>GATSCIQDEALNSEAAIDACTGDDVQLANINADSKLINVYVNKGADLSKQKLEFVIPEGATIKINDQVAGDTEATYDFSEETHSRKFTVTSEDGQWKPVYTVKVVLAELPTSFNFEELLPSNDYDIFYEFQPGTSQEISKVLQWSSGNPGFKLTGMANSKTDYPTVQVANGFRGKGVKLETRDTGSFGAMVKMYIAAGNLFIGTFEVGNALTDPRKATNFGFQFYKRP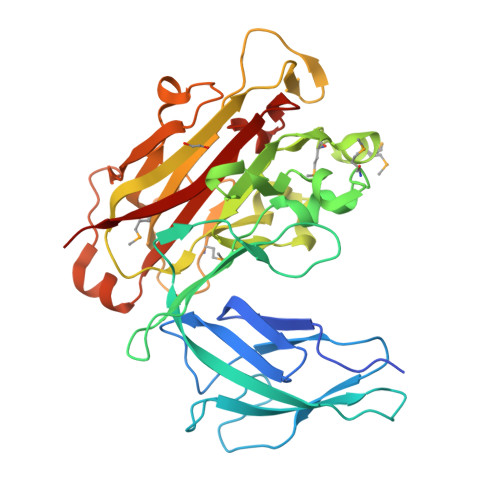KTLKGHYKFKAGDVYSVEGKPQEGVRDKCDIYAVMYEAENNSVMLNGDDVFTSDKLVSLARIKPEDVVESDQWTDFEIPFEPVKGRVIDDTKLKNGKYKLGIVLSSSVDGAYFKGAVGSTLYVDEVELICED[2x]>[4x]MRVLALSAVFLVASIIGMPAVAKEWQENKSWNAHFTEHKSQGV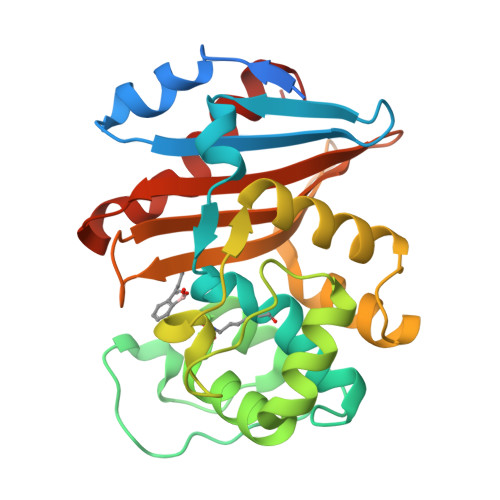VVLWNENKQQGFTNNLKRANQAFLPASTFKIPNSLIALDLGVVKDEHQVFKWDGQTRDIATWNRDHNLITAMKYSVVPVYQEFARQIGEARMSKMLHAFDYGNEDISGNVDSFWLDGGIRISATEQISFLRKLYHNKLHVSERSQRIVKQAMLTEANGDYIIRAKTGYSTRIEPKIGWWVGWVELDDNVWFFAMNMDMPTSDGLGLRQAITKEVLKQEKIIP Riboflavin is essential in all organisms as a precursor for flavocoenzymes. More specifically, LS catalyzes the condensation of 5-amino-6-ribityl­amino-2,4(1H,3H)-pyrimidinedione with 3,4-dihydroxy­butanone 4-phosphate (compound 2), affording 6,7-dimethyl-8-ribityllumazine (compound 3), and riboflavin synthase catalyzes the dismutation of two molecules of compound 3 to form one molecule each of riboflavin (compound 4) and compound 1. Catalysis occurs in equivalent active sites, which are located at the interfaces of adjacent subunits in the pentamers. Owing to the absence of the riboflavin-biosynthesis pathway in animals, the enzymes of the pathway are potential targets for anti-infective therapy and riboflavin-biosynthesis inhibitors should be exempt from target-related toxicity.

The BaLS monomer is comprised of 153 amino acids and shows the typical α/β/α-sandwich topology of known LS orthologues. The N-terminus of each subunit forms an extra β-strand extending to the β-sheet of the adjacent subunit. The symmetry-related α3 helices of each pentameric ensemble of icosahedral BaLS surround a central channel. The central part of the channel wall is formed by the side chains of five Lys97 residues, creating a positively charged patch whose charge is compensated by the side chains of Glu94. 12 pentameric blocks make up one icosahedral particle with a diameter of about 157 Å, which is rather similar to the previously determined sizes of icosahedral LSs [160 Å for LS from S. oleracea, 154 Å for LS from A. aeolicus and 156 Å for LS from B. subtilis]. The characteristic icosahedral ionic contacts described in detail by Zhang et al. are well conserved in the BaLS structure, although there is one fewer positively charged Arg residue compared with LS from the hyperthermophilic bacterium A. aeolicus. BaLS was crystallized from phosphate buffer. In the resulting structure, we found electron-density peaks at the 5σ level in each of the 90 active sites in the asymmetric unit. These densities were interpreted and refined as inorganic phosphate ions. The binding mode of the phosphate ion found in the BaLS structure is very similar to the phosphate-binding modes described in published LS structures.

>[90x]MVFEGHLVGTGLKVGVVVGRFNEFITSKLLGGALDGLKRHGVEENDIDVAWVPGAFEIPLIAKKMANSGKYDAVITLGTVIRGATTHYDYVCNEVAKGVASLSLQTDIPVIFGVLTTETIEQAIERAGTKAGNKGYESAVAAIEMAHLSKHWA>[8x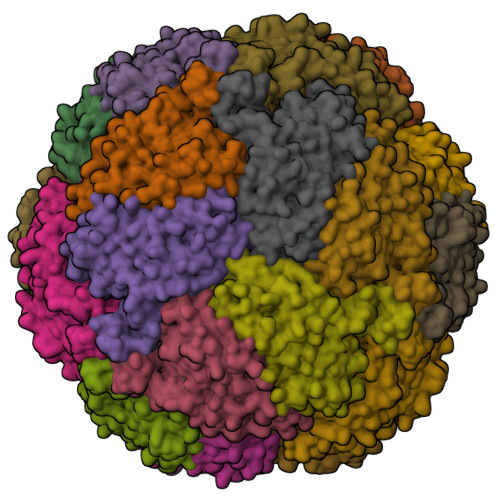]MPKPYVAINMVEVRNDPKTLELFGKVGPKVCMVTARHPGFVGFQNHVQIGVVPLGTRWGGAKMEMSQEMHSLMLMQYTFWKNWKDHEEMHKQNWANLFRLCLQCADQMIWGPYEPLYEIVYANMPLNTEMTDFTVMVGKKFAAGEAVSIPPISQPYGKRVVAFGEHIVKEGLENQFEEYAIKTLEAFRSAPGFLGGMILKEIGVSPLGSLQLNAKGFHQILETANGMDVPEPVTIYEAPEFRNRPQRYIVHTEWSDTNALMFGLGRVLIYPEVRQIHDKVLDTLVYGPYIRVLNPMMEGTYWREYLNEYHL methyl 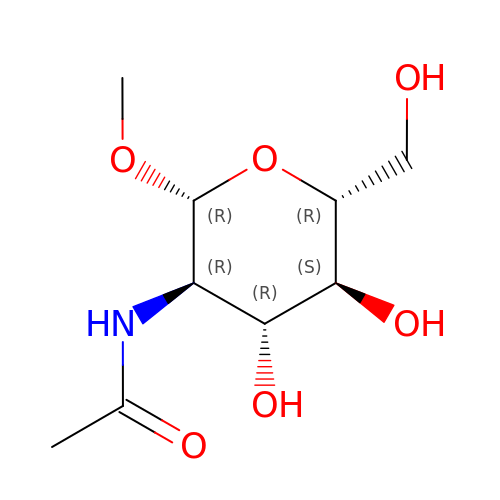2-acetamido-2-deoxy-beta-D-glucopyranoside | C9 H17 N O6 | ZEVOCXOZYFLVKN-JGKVKWKGSA-N> CPTHADSLNNLANIKREQGNIEEAVRLYRKALEVFPEFAAAHSNLASVLQQQGKLQEALMHYKEAIRISPTFADAYSNMGNTLKEMQDVQGALQCYTRAIQINPAFADAHSNLASIHKDSGNIPEAIASYRTALKLKPDFPDAYCNLAHCLQIVCDWTDYDERMKKLVSIVADQLEKNRLPSVHPHHSMLYPLSHGFRKAIAERHGNLCLDKINVLHKP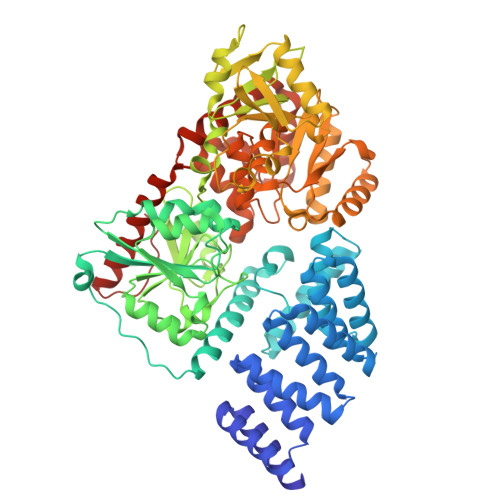PYEHPKDLKLSDGRLRVGYVSSNFGNHPTSHLMQSIPGMHNPDKFEVFCYALSPDDGTNFRVKVMAEANHFIDLSQIPCNGKAADRIHQDGIHILVNMNGYTKGARNELFALRPAPIQAMWLGYPGTSGALFMDYIITDQETSPAEVAEQYSEKLAYMPHTFFIGDHANMFPHLKKKAVIDFKSNGHIYDNRIVLNGIDLKAFLDSLPDVKIVKMKCPDGGDNADSSNTALNMPVIPMNTIAEAVIEMINRGQIQITINGFSISNGLATTQINNKAATGEEVPRTIIVTTRSQYGLPEDAIVYCNFNQLYKIDPSTLQMWANILKRVPNSVLWLLRFPAVGEPNIQQYAQNMGLPQNRIIFSPVAPKEEHVRRGQLADVCLDTPLCNGHTTGMDVLWAGTPMVTMPGETLASRVAASQLTCLGCLELIAKNRQEYEDIAVKLGTDLEYLKKVRGKVWKQRISSPLFNTKQYTMELERLYLQMWEHYAAGNKPDHMIKPVE>QAHHVSRNKRGQVVGTRGGFRGCTVWLTGLSGAGKTTISFALEEYLVSHAIPCYSLDGDNVRHGLNRNLGFSPGDREENIRRIAEVAKLFADAGLVCITSFISPF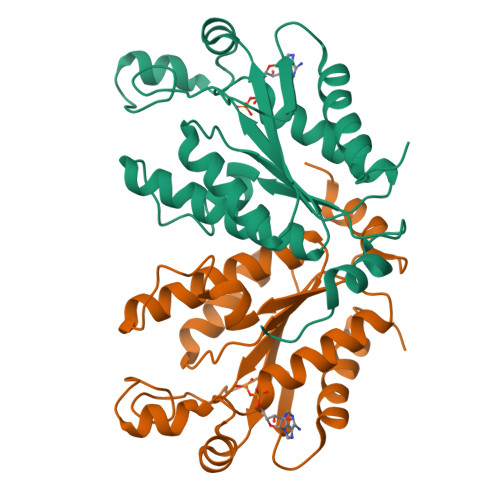AKDRENARKIHESAGLPFFEIFVDAPLNICESRDVKGLYKRARAGEIKGFTGIDSDYEKPETPERVLKTNLSTVSDCVHQVVELLQEQNIVPY[4x]> GPGSSDSKQHIEVLKESLTAKEQRAAILQTEVD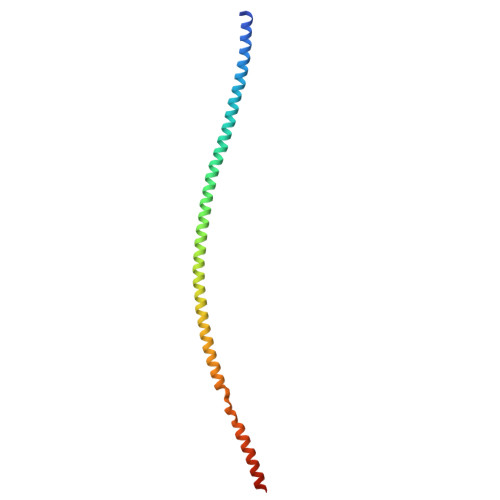ALRLRLEEKETMLNKKTKQIQDMAEEKGTQAGEIHDLKDMLDVKERKVNVLQKKIENLQEQLRDKEKQMSSLKERVKSLQADTTNTDTALTTLEEALADKERTIERLKEQRDR>[5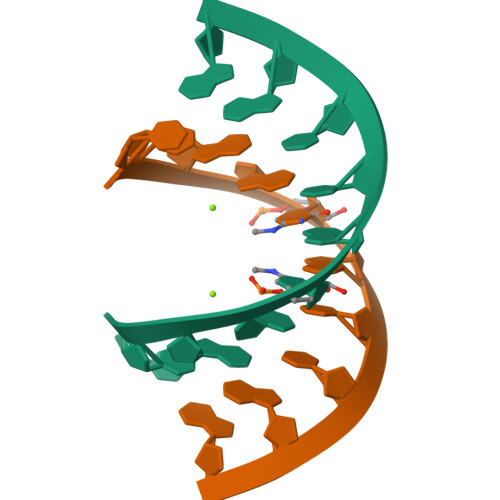x]CCGGCGCCGG>[2x]MATVKLSFLQHICKLTGLSRSGRKDELLRRIVDSPIYPTSRVLGIDLGIKNFSYCFASQNEDSKVIIHNWSVENLTEKNGLDIQWTEDFQPSSMADLSIQLFNTLHEKFNPHVILMERQRYRSGI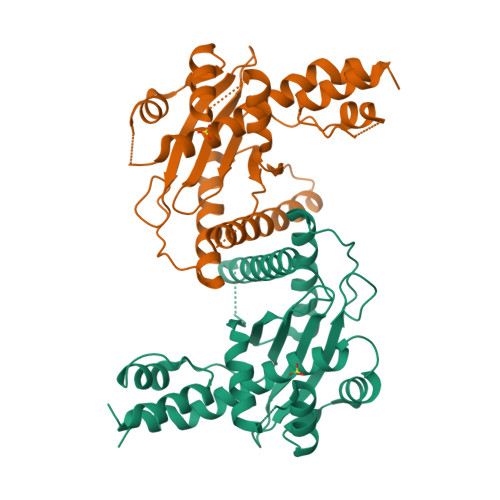ATIPEWTLRVNMLESMLYALHYAEKRNSIEQKIQYPFLLSLSPKSTYSYWASVLNTKASFSKKKSRVQMVKELIDGQKILFENEEALYKWNNGSRVEFKKDDMADSALIASGWMRWQAQLKHYRNFCKQFLKQ> MRRIRRPKVRIEIVTDDNTFTLRFEDTRDYNGDEFGAKLLGFQTKNSMEDDSSVFQINMAGDTYWDKLVMANDIIRIFITPNDDPNDKEGKQERLIQVGMVSQVSKVGSYGNDQTQFRITGQSFVKPFMKFGLGVIQEVQAVLPEVGWLIDGDGDNEVKFTGSSAHEVMTGIIRRFIPYMKYNYTEKTYNTIDNYLDYDDLSSWDEFEKLTEVSAFTNFDGSLKQLMDMVTARPFNELFFKNSEKTPGKAQLVLRKTPFNPTEWRALDMIKVPTEDFIEEDVGKSDVETYSIFTATPAGMLKELNGDVFSKPQFHPELTDR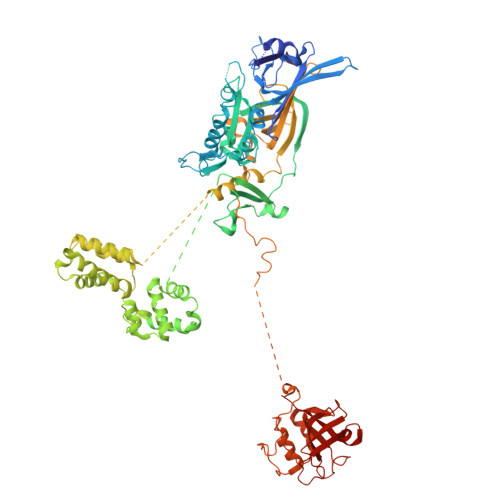YGYTKFEVENIYLSTKSGSATEDSDSSGDDNGTERGTYSKIMKDLSNYGRDNISKGIDKYTSKLSSKYKNLKKAQAKKIIEKFVKEGKVTEKEYEKITGNKVDDELTSDNRPKLTKDKLKSILKEKFKTQDDFNNSKKKKKAKTDALKELTTKYRFGNKTHATTLLDEYIKYKGEPPNDEAFDKYLKAIEGVSNVATDTGSDASDSPLVMFSRMLFNWYHGNPNFYAGDIIVLGDPKYDLGKRLFIEDKQRGDTWEFYIESVEHKFDYKQGYYTTVGVTRGLKDAILEDGKGSPHRFAGLWNQSSDFMGGLMGEDTSKELKEKGVAEKQSSGDKDGGSDSGGAQDGGSLDSLKKYNGKLPKHDPSFVQPGNRHYKYQCTWYAYNRRGQLGIPVPLWGDAADWIGGAKGAGYGVGRTPKQGACVIWQRGVQGGSPQYGHVAFVEKVLDGGKKIFISEHNYATPNGYGTRTIDMSSAIGKNAQFIYDKK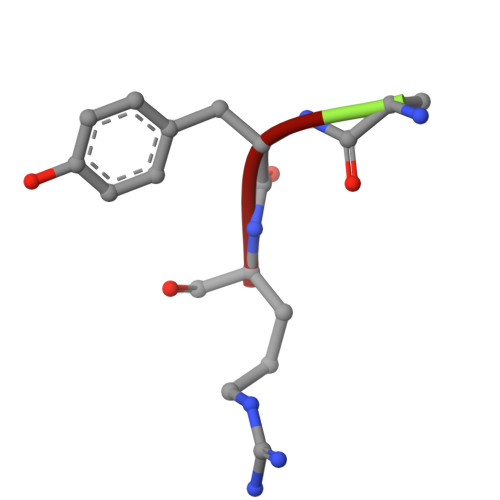> AYR> MAELAKSAVLVSSCTDDLLGDAKQVVVGPNQEDLHSAEAVLNRYSTVGFQASNLARAFSICEMMLTPQSPSPSLMPTEGDQASESPVMVQPTLFVGVTANLFGTGCREAIRFLCTECVPLPNGVEPATPLDDMAGISCDGTGALKPSPCDSRALIHVLVVSGGAMEHDIRRACESYKLSRDGAEEEGEQFHHPVERDRSRSKGTDCHFGNVRYNSSGVASRNLFSCVMRCLVKRLAEAQRKEKANREAAPIPEAYYD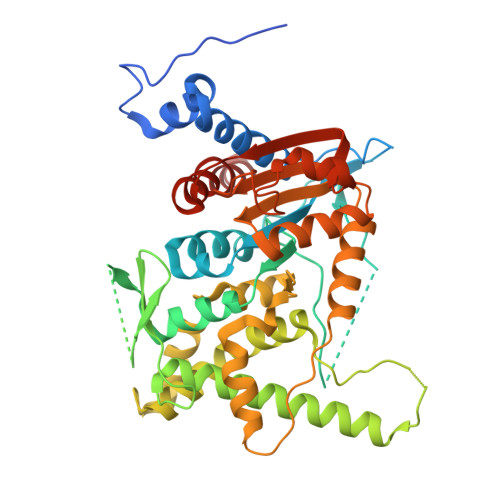VCSWAITPSTLWYMAGLWMADIFTEALQETGEVTDEKVASEEGLKRAKSTVLYWAARNGVPIFSPSLTDGDIMEFILTAGDTGVPLLQLDLVADIHRLNRLAMRSRRTGMMILGGGVVKHHVCNANLMRNGADYAVFLNNAQEFDGSDAGARPGEAVSWGKLRLDSTAVKVYSEVTIVFPLIVVHVFVAWVRMMRSKGKENIRS>CPRFLKVKNWETDVVLTDTLHLKSTLETGCTEHICMGSIMLPSQHTRKPEDVRTKDQLFPLAKEFLDQYYSSIKRFGSKAHMDRLEEVNKEIESTSTYQLKDTELIYGAKHAWRNASRCVGRIQWSKLQVFDARDCTTAHGMFNYICNHVKYATNKGNLRSAITIFPQRTDGKHDFRVWNSQLIRYAGYKQPDGSTLGDPANVQFTEICIQQGWKAPRGRFDVLPLLLQANGNDPELFQIPPELVLEVPIRHPKFDWFKDLGLKWYGLPAVSNMLLEIGGLEFSACPFSSWYMGTEIGVRDYCDNSRYNILEEVAKKMDLDMRKTSSLWKDQALVEINIAVLYSFQSDKVTIVDHHSATESFIKHMEN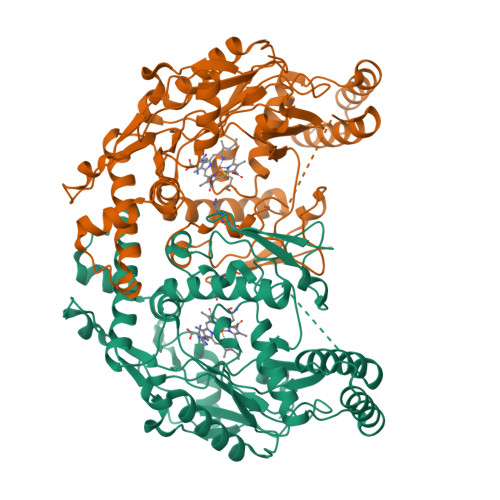EYRCRGGCPADWVWIVPPMSGSITPVFHQEMLNYRLTPSFEYQPDPWNTHVWKG[2x]>[4x]HPG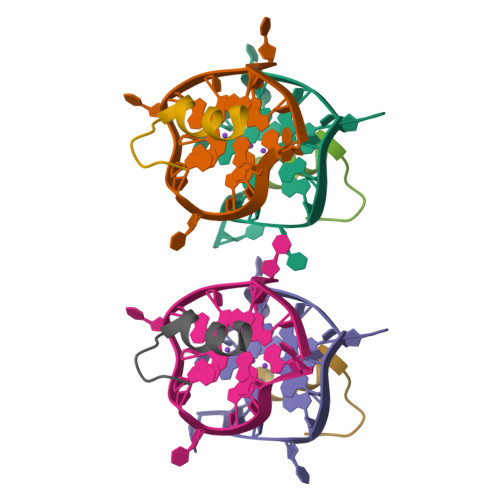HLKGREIGMWYAKKQGQKNKEAERQE(2R)-3-{[(BENZYLAMINO)CARBONYL]AMINO}-2-HYDROXYPROPANOIC ACID | C11 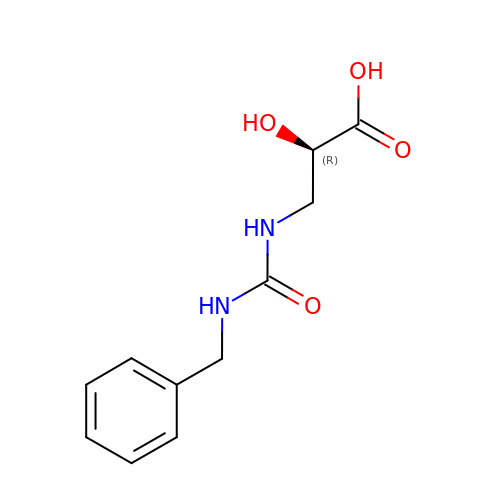H14 N2 O4 | KGFDIRSBGRVEFZ-SECBINFHSA-N> GSEFVKEHDWKKCDQSGFCRRNRAYADHALSAISWESPYKIAPETGSFKDGQYQAIILKTINDHGETVRLPLTVSFLESGTARVTIDEEKRQKGEIELRHDSKARKERYNEAEQWVIVGGMTLDKGAKVDYEDKTQMTVKYGPSSKFEATIKFAPFSIDFKRDGASHIKFNDQGLLNIEH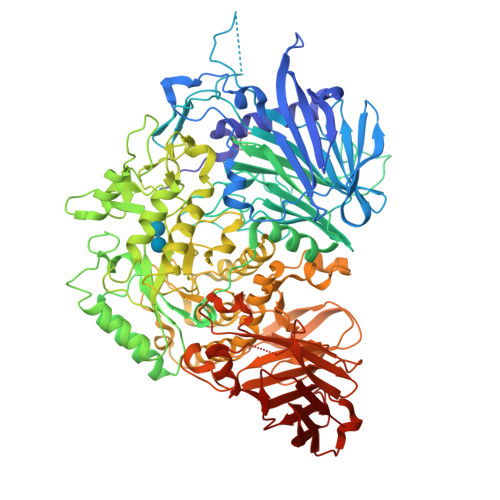WRPKIDPPPEPEKKEGEQQPDKKEEAPREDDSTWWEESFGGNTDSKPRGPESVGLDISFVGYEHVFGIPSHASPLSLKQTRGGEGNYNEPYRMYNADVFEYILDSPMTLYGSIPFMQAHRKDSSVGIFWLNAAETWVDITKGKDSKNPLALGVKSKITTRTHWFSESGLLDVFVFLGPTPKDIISKYAELTGTTAMPQEFSLGYHQCRWNYVSDEDVKDVDRKMDKFNMPYDVIWLDIEYTDEKKYFTWDKHSFKDPIGMGKQLEAHGRKLVTIIDPHIKNTNNYPVVDELKSKDLAVKTKDGSIFEGWCWPGSSHWIDAFNPAAREWWKGLFKYDKFKGTMENTFIWNAMNEPSVFNGPEVTMPKDNLHHGNWEHRDVHNLNGMTFQNATYHALLSRKPGEHRRPFVLTRAFFAGSQRLGAMWTGDNTADWGYLKASIPMVLSQGIAGFPFAGADVGGFFGNPDKDLLTRWYQTGIFYPFFRAHAHIDARRREPYLTGEPYNTIIAAALRLRYSLLPSWYTAFRHAHLDGTPIIKPMFYTHPSEEAGLPIDDQFFIGNTGLLAKPVTDKDRTSVDIWIPDSEVYYDYFTYDIISAAKSKTATLDAPLEKIPLLMRGGHVFARRDIPRRSSALMKWDPYTLVVVLGNDRKAEGDLYVDDGDSFDYEKGQYIHRRFIFDANTLTSADYEGRDDASIKEGEWLKKMRTVNVEKIIVVGAPAAWKGKKTVTVESEGKTWAAAIEYNPAEKSRAAFAVVKKVGVRVGADFKIVFG> MASSSHNPVILLKRILSLTESSPFILCLD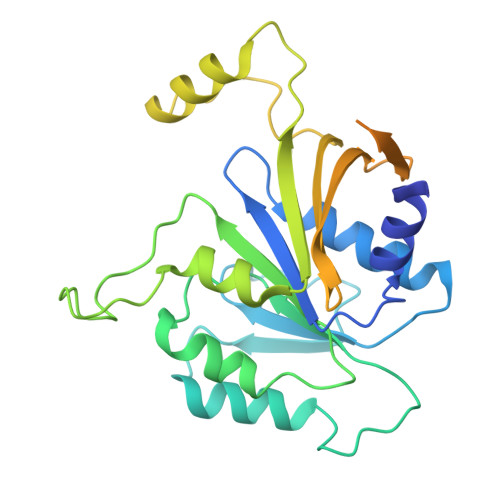SIAQTSYKLIQEFVHQSKSKGNEYPIVYISFETVNKPSYCTQFIDATQMDFVHLVKQIISYLPAATATQAKKHMVIIDSLNYISTEYITRFLSEIASPHCTMVATYHKDIKDENRTVIPDWNNNYPDKLTLLQFMATTIVDIDVVLTGTLDTEEVSELLNEFRIPRGLNNDIFQLRLVNKRKSGRSLEYDFIVNSNTHEYELLSTTKQEEESSSNGLETPEMLQGLTTFNLGTSNKQKLAKDQVALPFLEAQSFGQGGAIVYEYEKDDDYDEEDPYEDPF> TR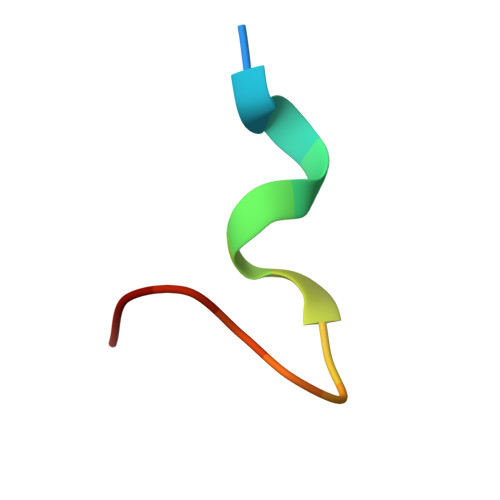YANAKMLPFAFGA>[3x]MKCLFYIAGDVSNYSIVNYELNGQTQNTFFAAHALYNLFKPDKVIALIPDSLVKDNVSDEECYKN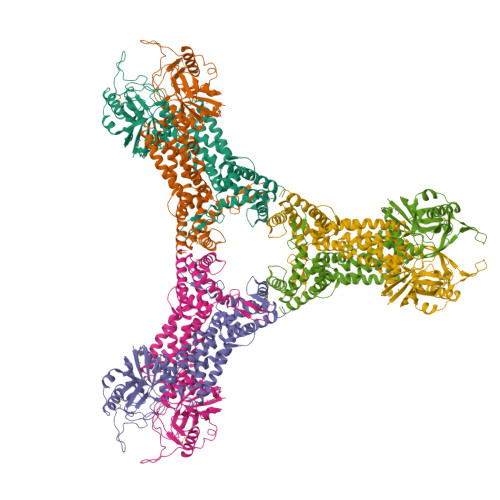LVINRAKELNFAGMEEFMNKVEIRKIPNVGIASAIQCENGAPKKEKNKEGREVLKRLPYNEKRSPIFIFNAIYAIFKDEACDEYLVDLTHGTNVLVSIGMNVGALFNAKFYSAPVMGMPGKDSIVNIVELTDVVQATNDSLMIRSSIENLDERYFKDYSAKLSRLNPTIFEEEEKKVLTRVKGTDVNVVINFLWNIRNGFTVNAVKSMNELKNIINQLEEDLEKLKSFYKNWEEHKNFQGETLLVLSDLDSTLKVKDLLIEGNDLEKLNYLLDLYIKASIYDKALSLARELPVAICLNKVGGGMFDDKNEKYKHCNEIVTSYLRLRYSGLMEFRNTLMHGGLSTDMKPNVDKDGNITPGKIVTKNKIEDFVKRELRNYFDKIVNFLSSA2,6-DIFLUOROPHENOL 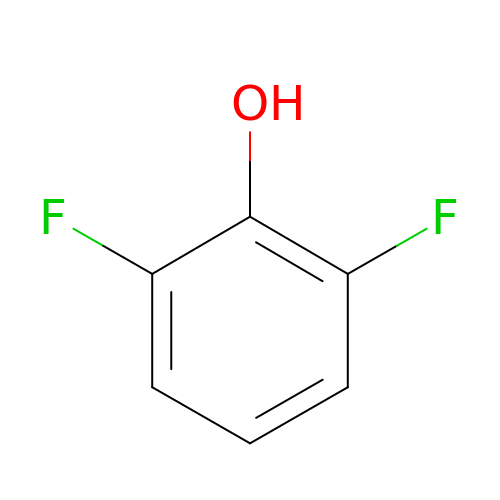| C6 H4 F2 O | CKKOVFGIBXCEIJ-UHFFFAOYSA-N>[6x]GSGSDSFINVINTLGRNDGAKYIGECHSVADLRNTEPTMDGQRIILKQHTAGTLLGGGVFRALIDGTGKTDNNGTVIKTVGGAAWLRVNADRVNPFMFGALGGSNDDTIPVQSCVDSGKATQLTDAHYVSNIQLKYNTSSIYGSGLHYSRLHQLPSATGNCITIKDTCSLIVLDAFGVYGTGAQQGTSFTAGTTGIYVETPSGLSADYPFHTTADPRRDLCISKVHIAGFDEYGLNIDSGNFSVTTDSLLVNHINQVGVRCATTDWT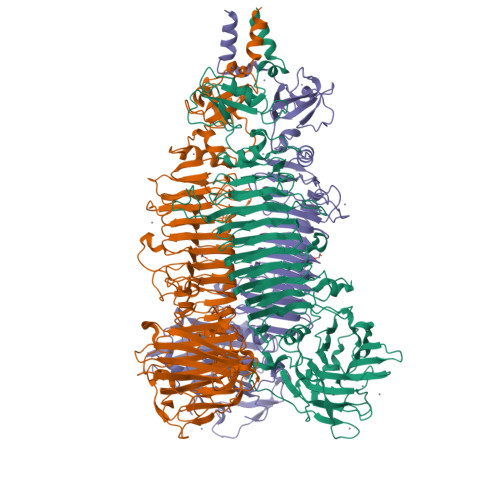WTNIQVNTCGKQCLVLDGCGNGRIIGGKFIWANWQPYGTVGQFPGITINNSQNMVINGIEVQDCGGNGIEISESYSISMNGLNTNRNGINANNTFYNIVFNKSDAVINGFVGLNYAANSGSGANSSAGNFQFLSNDCSVTINGVVETGYMGINFIGDNNIINPTNSDLSINGLVNYSKTGLQTMNETPTFDGVSTTPVYVSVPSSVGQVNGLRLSQANKDKLLYSRTAGPEGITMAAVIVPTISGAEVFNFMAIGSGFSDTSNSLHLQLVIDASGKQTIALLLGGDGTTQILSGDLPNDLKLQSGVPYHIAIGAKPGYFWWSILNIQTGKRIRRSFRGAYLAVPFNSIFGLTSSLTFFSDSNAGGDACSGVGAKVYVGMFSSENDYVASRYYNLINPVDPTKLISYRILDSSI>[2x]MLSVAGHRFASLATTPVLRMGLARCFSSVTGPFQCPPLPYVKNALEPHMSAETLTYHHDKHHQTYVDTLNSIAAENSTIASKTLEQIIKTETGKPFNQAAQVYNHTFFFNNLA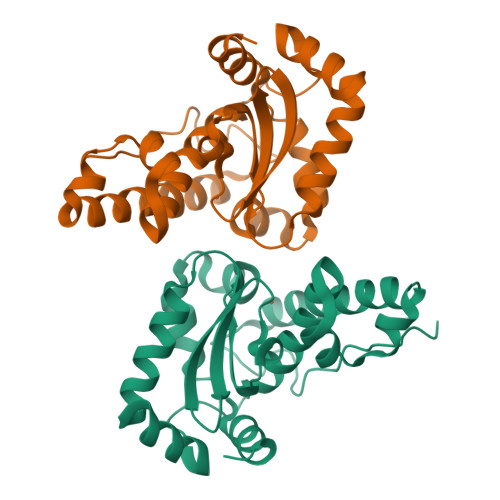PNGGGEPTGKIAELITRDFGSFEKFKEDFSAAAVGHFGSGWVWLIADDGKLKIVQGHDAGNPIRESKTPLMNIDVWEHAYYIDYRNARAQYVKNYWNLVNWDFVNDNVAKAGI>[4x]GSMAGKE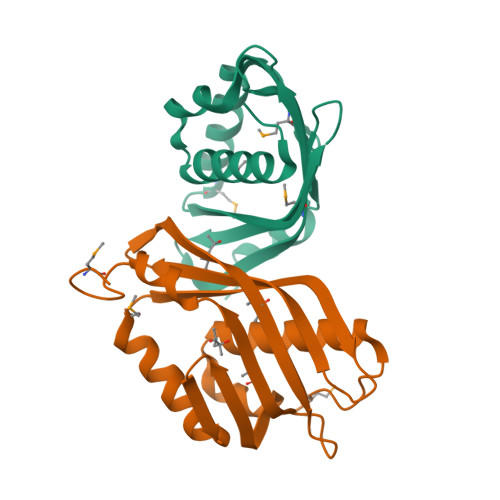IQTPDQAEAFVAKVFDVLDSYDYTRFGEVLSTDLKYEGGLQKTSGLDNFINDIKASTQRMPGLQTSHSRYRTELTAEGTIYSEGHSNASLESNPGKVVTVPMIGVFKLDSEDGKIKEMRIYKDRLPFLALHQALPGMKANN> MYPVDLHMHTVASTHAYSTLSDYIAQAKQKGIKLFAITDHGPDMEDAPHHWHFINMRIWP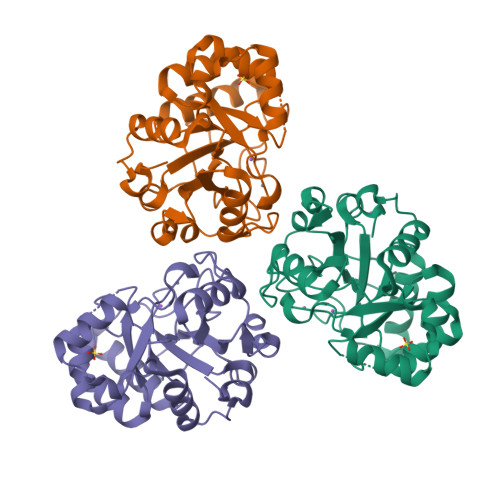RVVDGVGILRGIEANIKNVDGEIDCSGKMFDSLDLIIAGFHEPVFAPHDKATNTQAMIATIASGNVHIISHPGNPKYEIDVKAVAEAAAKHQVALEINNSSFLHSRKGSEDNCREVAAAVRDAGGWVALGSDSHTAFTMGEFEECLKILDAVDFPPERILNVSPRRLLNFLESRGMAPIAEFADL>[2x]NLSDDLSFNFDKFVPNQKNIIFQGDASVSTTGVLQVTKVSKPTTTSIGRALYAAPIQIWDSITGKVASFATSFSFVVKADK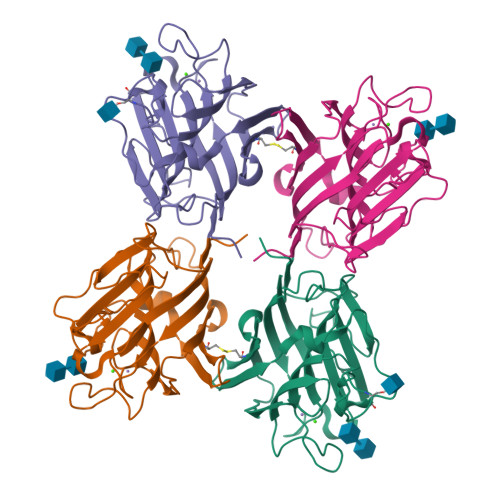SDGVDGLAFFLAPANSQIPSGSSAGMFGLFSSSDSKSSNQIIAVEFDTYFGKAYNPWDPDFKHIGIDVNSIKSIKTVKWDWRNGEVADVVITYRAPTKSLTVCLSYPSDGTSNIITASVDLKAILPEWVSVGFSGGVGNAAEFETHDVLSWYFTSNLEANN>FNKIKDSVKQKIDSMGDKGTYGVSASHPLAVEEGMKVLKNGGSAVDAAIVVSYVLGVVELHASGIGGGGGMLIISKDKETFIDYRETTPYFTGNQKPHIGVPGFVAGMEYIHDNYGSLPMGELLQPAINYAEKGFKVDDSLTMRLDLAKPRIYSDKLSIFYPNGEPIETGETLIQTDLARTLKKIQKEGAKGFYEGGVARAISKTAKISLEDIKGYKVEVRKPVKGNYMGYDVYTAPPPFSGVTLLQMLKLAEKKEVYKDVDHTATYMSKMEEISRIAYQDRKKNLGDPNYVNMDPNKMVSDKYISTMKNENGDALSEAEHES[2x];>[2x]TTHFVIIDRDGTVVSSTNTLSNFFGTGKYTAGFFLNNQLQNFGSEGFNSYEPGKRSRTFMAPTVLKKDGETIGIGSPGGNRIPQILTPILDKYTHGK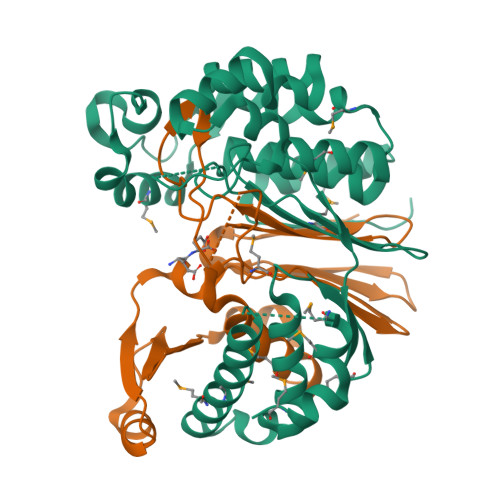GSLQDIINEYRFTFEKNTAYTEIQLSSEVKNELSRKGLNVKKKVSPAFFGGVQALIKDERDNVITGAGDGRRNGTWKSNK2',6'-DICHLORO-BIPHENYL-2,6-DIOL | C12 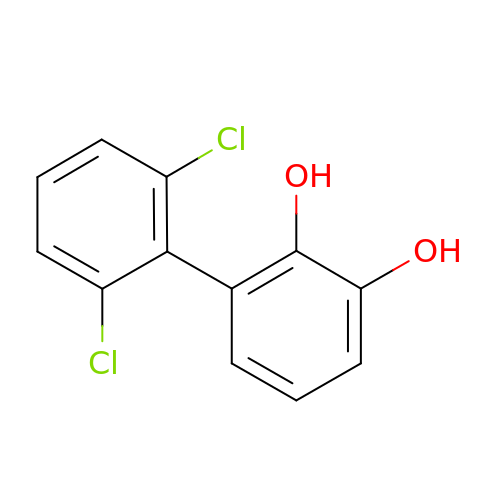H8 Cl2 O2 | MCZUCSAAGDCHHN-UHFFFAOYSA-N>TYKITVRVYQTNPDAFFHPVEKTVWKYANGGTWTITDDQHVLTMGGS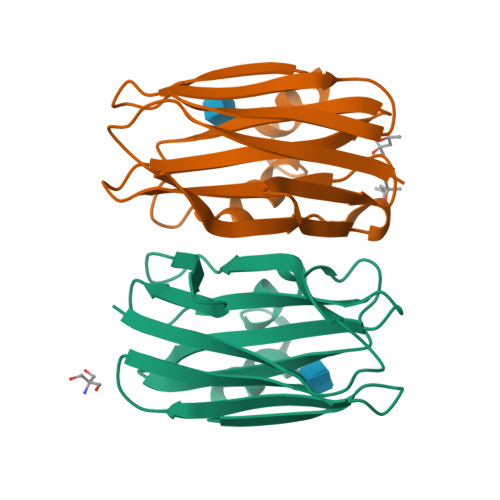GTSGTLRFHADNGESFTATFGVHNYKRWCDIVTNLAADETGMVINQQYYSQKNREEARERQLSNYQVKNAKGRNFQIVYTEAEGNDLHANLIIG[2x]2,6-DIAMINO-3H-QUINAZOLIN-4-ONE | C8 H8 N4 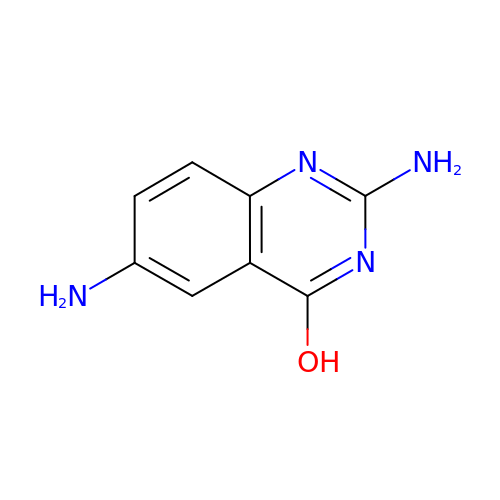O | YCRCNZBZUQLULA-UHFFFAOYSA-N(2Z)-2-(3-amino-1H-isoindol-1-ylidene)hydrazine-1-carboximidamide | 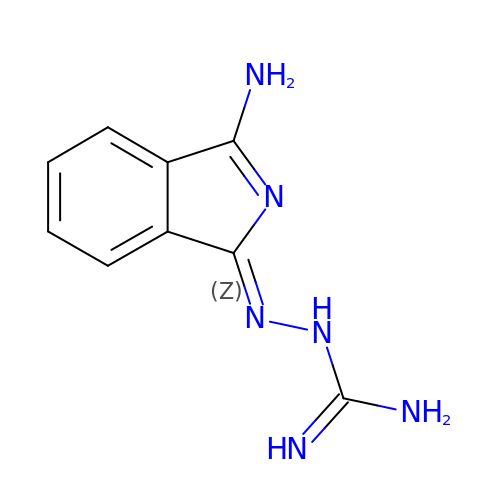C9 H10 N6 | MMCURALNZRAPHY-UHFFFAOYSA-N>[2x]MARKTKEDTQATREGILDAAEACFHEHGVARTTLEMIGARAGYTRGAVYWHFKNKSEVLAAIVERVHL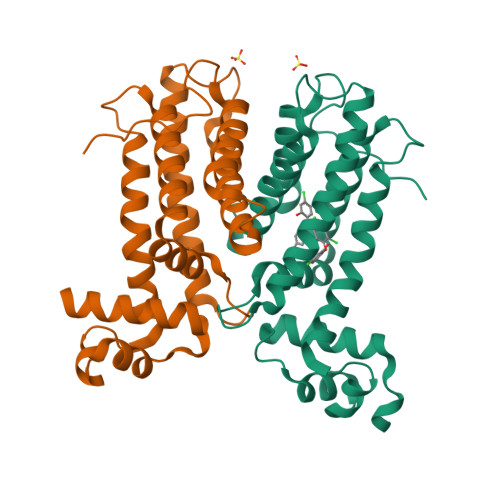PFMQELERTSTDQRDTPVHDLRAVMIHSFIELSEDERLRKTMEIMLRSDASANTRVLTEMQQAGFRDALDRMERALRRARDLGQLREGADPKIAARMLHATVLGVLHGAMVEPELMDLKRDGMLALDMTLAAYVKDGVFVPGTVPEPLPEA> PSFDCGKPQVEPKKCPGRVVGGCVAHPHSWPWQVSLRTRFGMHFCGGTLISPEWVLTAAHCLEKSPRPSSYKVILGAHQEVNLEPHVQEIEVSRLFLEPTRKDIALLKLSSPAVITDKVIPACLPSPNYVVADRTECFITGWGETQGTFGAGLLKEAQLPVIENKVCNRYEFLNGRVQSTELCAGHLAGGTDSCQGDAGGPLVCFEKDKYILQGVTSWGLGCARPNKPGVYVRVSRFVTWIEGVMRNN;> MIAGPEALLDRPSVNNSQLVVSVAGTVEGTNQDISLKFFEIDLTSRPASKPFATDSGAMPHKLEKADLLKA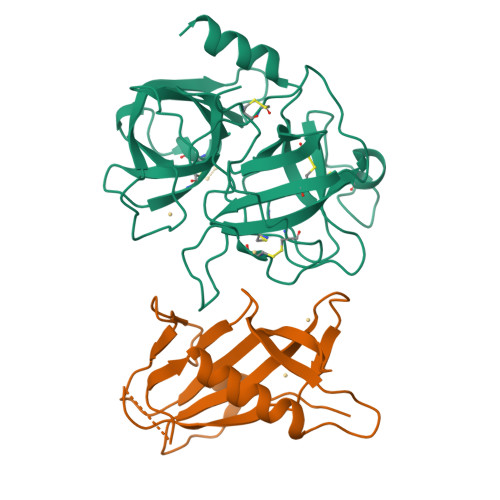IQEQLIANVHSNDDYFEVIDFASDATITDRNGKVYFADKDGSVTLPTQPVQEFLLSGHVRVRPYK>[2x]MKPTHWGA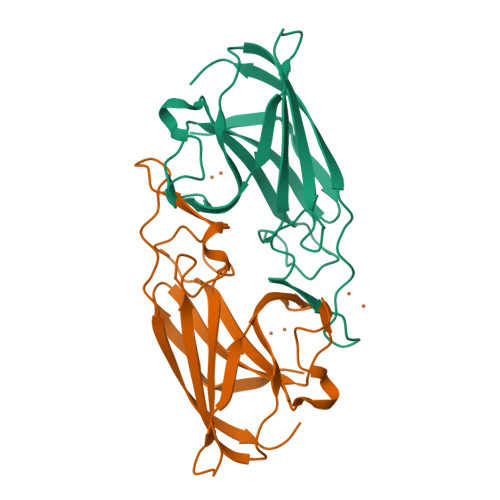ALALAAACFTTSAYALEYPIGTPQNLAGMEIAAVYLQPIDMEPEGHMRKASESDIHIEADIHALSNNPNGYPEGFWVPFLFIKYEITKVGGSGAPITGDMMAMVASDGPHYGDNVKLQGPGKYKVKYTIYPPNAKENPMSPYYGRHTDRETGVRPWFKTFSVEWDFTYAGIGKKGGYSWSHPQFEK> GSSPEGGEDSDRE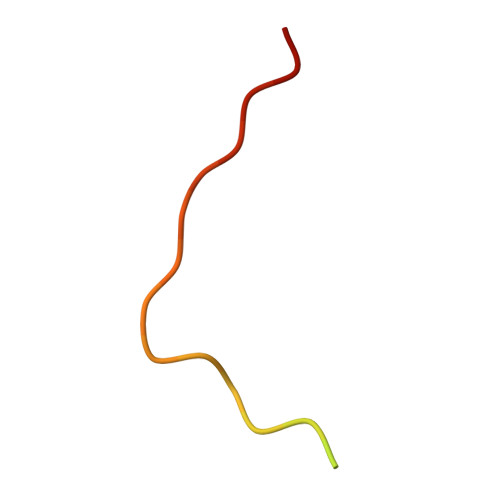DGNYCPPVKRERTSSLT{6-[(4-methoxyphenyl)amino]-1-benzofuran-3-yl}acetic acid | C17 H15 N O4 | 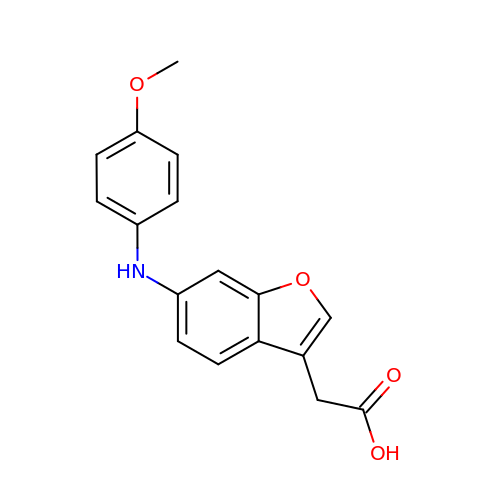MFCXHNGDMBSNNX-UHFFFAOYSA-N2-[[(E,2S,3R)-2-(hexanoylamino)-3-oxidanyl-dec-4-enoxy]-oxidanyl-phosphoryl]oxyethyl-trimethyl-azanium 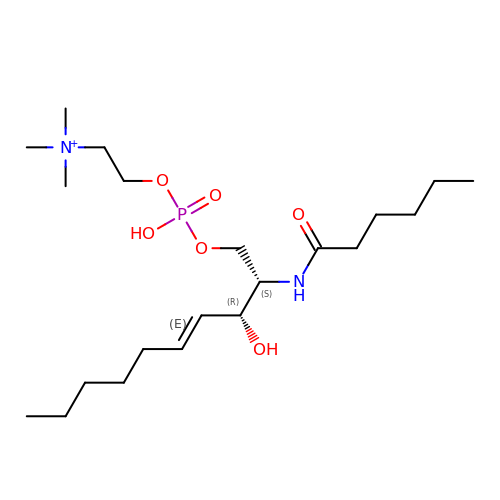| C21 H44 N2 O6 P | XVUOEYGVFVFEDQ-FGXJKGHSSA-O>[2x]MSTDDGRRPIRRALISVYDKTGLVDLAQGLSAAGVEIISTGSTAKTIADTGIPVTPVEQLTGFPEVLDGRVKTLHPRVHAGLLADLRKSEHAAALEQLGIEAFELVVVNLYPFSQTVESGASVDDCVEQIDIGGPAMVRAAAKNHPSAAVVTDPLGYHGVLAALRAGGFTLAERKRLASLAFQHIAEYDIAVASWMQQTLAPEHPVAAFPQWFGRSWRRVAMLRYGENPHQQAALYGDPTAWPGLAQAEQLHGKDMSYNNFTDADAAWRAAFDHEQTCVAIIKHANPCGIAISSVSVADAHRKAHECDPLSAYGGVIAANTEVSVEMAEYVSTIFTEVIVAPGYAPGALDVLARKKNIRVLVAAEPLAGGSELRPISGGLLIQQSDQLDAHGDNPANWTLATGSPADPATLTDLVFAWRACRAVKSNAIVIAADGATVGVGMGQVNRVDAARLAVERGGERVRGAVAA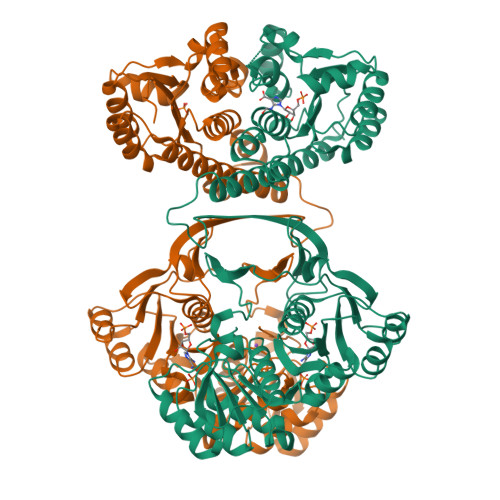SDAFFPFPDGLETLAAAGVTAVVHPGGSVRDEEVTEAAAKAGVTLYLTGARHFAH>[2x]MKGTLVGTWIKTLRDLYGNDVVDESLKSVGWEPDRVITPLEDIDDDEVRRIFAKVSEKTGKNVNEI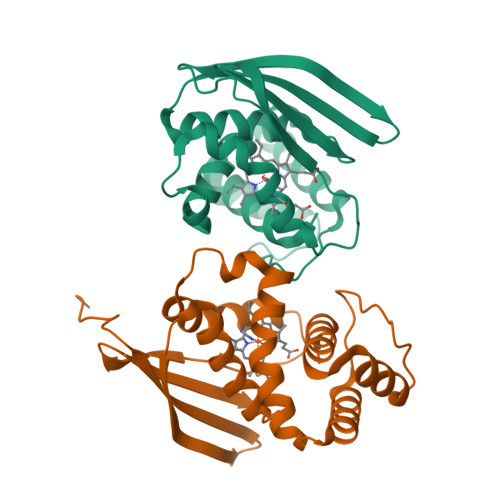WREVGRQNIKTFSEWFPSYFAGRRLVNFLMMMDEVHLQLTKMIKGATPARLIAKPVAKDAIEMEYVSKRKMYDYFLGLIEGSSKFFKEEISVEEVERGEKDGFSRLKVRIKFKNPVFEYKKN>GIPRNSLEKFNVDLMKKAGKELGLSLSPNEIGCTIADLIQGQYPEIDSKLQRGDIITKFNGDAL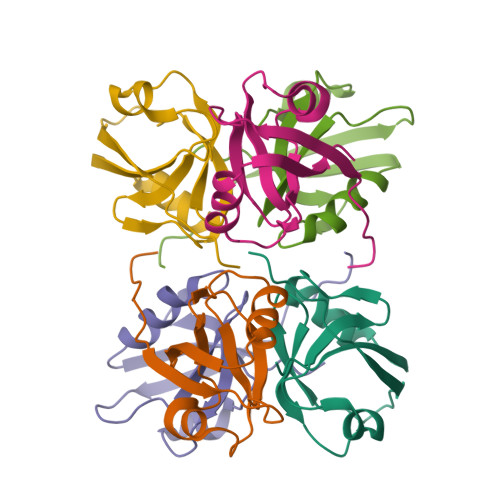EGLPFQVSYALFKGANGKVSMEVTRPKPAAAS[2x]>MGFKSWITEKLNPGQRIIRDMEPVSHRTNRKPFTTGQAYSKIEILNRTANMVIDSAAECSYTVGDKYNIVTYANGVKTKTLDTLLNVRPNPFMDISTFRRLVVTDLLFEGCAYIYWDGTSLYHVPAALMQVEADANKFIKKFIFNNQINYRVDEIIFIKDNSYVCGTNSQISGQSRVATVIDSLEKRSKMLNFKEKFLDNGTV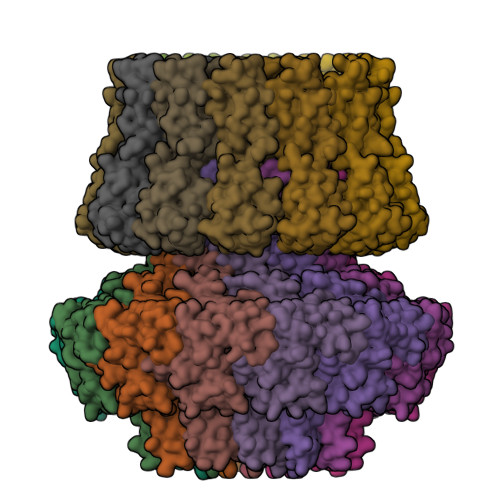IGLILETDEILNKKLRERKQEELQLDYNPSTGQSSVLILDGGMKAKPYSQISSFKDLDFKEDIEGFNKSICLAFGVPQVLLDGGNNANIRPNIELFYYMTIIPMLNKLTSSLTFFFGYKITPNTKEVAALTPDKEAEAKHLTSLVNNGIITGNEARSELNLEPLDDEQMNKIRIPANVAGSATGVSGQEGGRPKGSTEGD[12x];>[12x]MQIITAEDYRLYGGLKRPELESGVEVMITAANALITSLLGMDDADAVDQLITTKPTRKKYFLSSPSATSVTKMTINDKEIDPEQYKLYSDGVILLKFNPPEGYMDVEYTQGGFNPMPEDLKLAACMLVDHWHKQDYRQARTIGGETVTFNNTKSGIPEHIRTIIEVYRRV> MASPRSSGQPGPPPPPPPPPARLLLLLLLPLLLPLAPGAWGWARGAPRPPPSSPPLSIMGLMPLTKEVAKGSIGRGVLPAVELAIEQIRNESLLRPYFLDLRLYDTECDNAKGLKAFYDAIKYGPNHLMVFGGVCPSVTSIIAESLQGWNLVQLSFAATTPVLADKKKYPYFFRTVPSDNAVNPAILKLLKHYQWKRVGTLTQDVQRFSEVRNDLTGVLYGEDIEISDTESFSNDPCTSVKKLKGNDVRIILGQFDQNMAAKVFCCAYEENMYGSKYQWIIPGWYEPSWWEQVHTEANSSRCLRKNLLAAMEGYIGVDFEPLSSKQIKTISGKTPQQYEREYNNKRSGVGPSKFHGYAYDGIWVIAKTLQRAMETLHASSRHQRIQDFNYTDHTLGRIILNAMNETNFFGVTGQVVFRNGERMGTIKFTQFQDSREVKVGEYNAVADTLEIINDTIRFQGSEPPKDKTIILEQLRKISLPLYSILSALTILGMIMASAFLFFNIKNRNQKLIKMSSPYMNNLIILGGMLSYASIFLFGLDGSFVSEKTFETLCTVRTWILTVGYTTAFGAMFAKTWRVHAIFKNVKMKKKIIKDQKLLVIVGGMLLIDLCILICWQAVDPLRRTVEK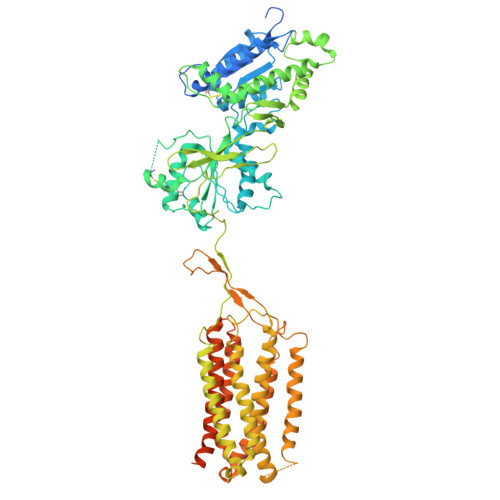YSMEPDPAGRDISIRPLLEHCENTHMTIWLGIVYAYKGLLMLFGCFLAWETRNVSIPALNDSKYIGMSVYNVGIMCIIGAAVSFLTRDQPNVQFCIVALVIIFCSTITLCLVFVPKLITLRTNPDAATQNRRFQFTQNQKKEDSKTSTSVTSVNQASTSRSGRGGSENLYFQGGSGSGGDYKDDDDKDYKDDDDK>[2x]MVLYFIGLGLYDERDITVKGLEIAKKCDYVFAEFYTSLMAGTTLGRIQKLIGKEIRVLSREDVELNFENIVLPLAKENDVAFLTPGDPLVATTHAELRIRAKRAGVESYVIHAPSIYSAVGITGLHIYKFGKSATVAYPEGNWFPTSYYDVIKENAERGLHTLLFLDIKAEKRMYMTANEAMELLLKVEDMKKGGVFTD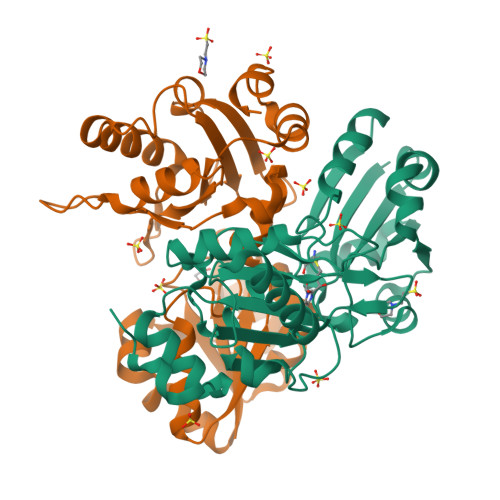DTLVVVLARAGSLNPTIRAGYVKDLIREDFGDPPHILIVPGKLHIVEAEYLVEIAGAPREIMRVNV>MDFSRNLYDIGEQLDSEDLASLKFLSLDYIPQRKQEPIKDALMLFQRLQEKRMLEESNLSFLKELLFRINRLDLLITYLNTRKEEMERELQTPGRAQISAYRVMLYQISEEVSRSELRSFKFLLQEEISKCKLDDDMNLLDIFIEMEKRVILGEGKLDILKRVCAQINKS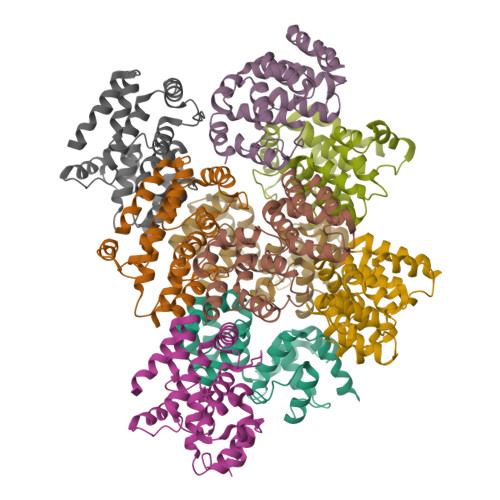LLKIINDYEEFSKE[9x]L and P function as the RNA polymerase complex, responsible for replicating and transcribing the viral genome. To catalyze the RNA synthesis in both replication and transcription, L sequentially consists of five domains: the RNA-dependent RNA polymerase domain (RdRp), polyribonucleotidyl transferase domain (PRNTase), connector domain (CD), methyltransferase domain (MTase), and C-terminal domain (CTD). P harbors an oligomerization domain (POD) for self-oligomerization, and the oligomeric P attaches to RdRp of L, tethering the polymerase to NC to extract the RNA strand for both replication and transcription. Here, we resolved two L–P complex conformations from the mumps virus (MuV), a typical member of nsNSVs, via cryogenic-electron microscopy.

RdRp-PRNTase is quite conserved in structure amongst nsNSVs, while CD-MTase-CTD resembles an appendage of RdRp-PRNTase with great structural diversity. In MuV Lintegral–P, the appendage is also less resolved compared with the body. Different from the conserved RdRp-PRNTase, CD-MTase-CTD of MuV Lintegral–P adopts a spatial organization distinct from those of PIV-5, though their individual structures are pretty similar. The detailed alignment showed that MTase and CTD in MuV Lintegral–P appears as an integral on the PRNTase side instead of the RdRp side compared with PIV-5 L. The overall spatial organization of CD-MTase-CTD in MuV Lintegral–P is surprisingly similar to VSIV L. VSIV CD-MTase-CTD is highly flexible unless unphosphorylated P locks their configuration, while in MuV, no P fragment is resolved around the appendage. In MuV Lintegral–P, an α-helix hinge termed Hinge-1 (L1416–1431) connecting PRNTase and CD has been visualized. It is supposed to provide flexibility to CD positioning via loops flanking it. Compared with PIV-5, the spatial organization of MuV CD-MTase-CTD renders the helices α53 (L1439–1458) and α57 (L1535–1544) of CD rotating upward and leaves more space for RNA to access MTase. Actually, MuV Lintegral–P forms a continuous positively-charged tunnel from the GDN to the K-D-K-E motifs, ideal for the RNA synthesis followed by 5’ capping and methylation, which is favorable as the transcription state.

> MAGLNEILLPEVHLNSPIVRYKLFYYILHGQLPNDLEPDDLGPLANQNWKAIRAEESQVHARLKQIRVELIARIPSLRWTRSQREIAILIWPRILPILQAYDLRQSMQLPTVWEKLTQSTVNLISDGLERVVLHISNQLTGKPNLFTRSRAGQDTKDYSIPSTRELSQIWFNNEWSGSVKTWLMIKYRMRQLITNQKTGELTDLVTIVDTRSTLCIITPELVALYSSEHKALTYLTFEMVLMVTDMLEGRLNVSSLCTASHYLSPLKKRIEVLLTLVDDLALLMGDKVYGIVSSLESFVYAQLQYGDPVIDIKGTFYGFICNEILDLLTEDNIFTEEEANKVLLDLTSQFDNLSPDLTAELLCIMRLWGHPTLTASQAASKVRESMCAPKVLDFQTIMKTLAFFHAILINGYRRSHNGIWPPTTLHGNAPKSLIEMRHDNSELKYEYVLKNWKSISMLRIHKCFDASPDEDLSIFMKDKAISCPRQDWMGVFRRSLIKQRYRDANRPLPQPFNRRLLLNFLEDDRFDPIKELEYVTSGEYLRDPEFCASYSLKEKEIKATGRIFAKMTKRMRSCQVIAESLLANHAGKLMRENGVVLDQLKLTKSLLTMNQIGIISEHSRRSTADNMTLAHSGSNKHRINNSQFKKNKDNKHEMPDDGFEIAACFLTTDLTKYCLNWRYQVIIPFARTLNSMYGIPHLFEWIHLRLMRSTLYVGDPFNPPSDPTQLDLDTALNDDIFIVSPRGGIEGLCQKLWTMISISTIILSATEANTRVMSMVQGDNQAIAITTRVVRSLSHSEKKEQAYKASKLFFERLRANNHGIGHHLKEQETILSSDFFIYSKRVFYKGRILTQALKNVSKMCLTADILGDCSQASCSNLATTVMRLTENGVEKDLCYFLNAFMTIRQLCYDLVFPQTKSLSQDITNAYLNHPILISRLCLLPSQLGGLNFLSCSRLFNRNIGDPLVSAIADVKRLIKAGCLDIWVLYNILGRRPGKGKWSTLAADPYTLNIDYLVPSTTFLKKHAQYTLMERSVNPMLRGVFSENAAEEEEELAQYLLDREVVMPRVAHVILAQSSCGRRKQIQGYLDSTRTIIRYSLEVRPLSAKKLNTVIEYNLLYLSYNLEIIEKPNIVQPFLNAINVDTCSIDIARSLRKLSWATLLNGRPIEGLETPDPIELVHGCLIIGSDECEHCSSGDDKFTWFFLPKGIRLDDDPASNPPIRVPYIGSKTDERRVASMAYIKGASVSLKSALRLAGVYIWAFGDTEESWQDAYELASTRVNLTLEQLQSLTPLPTSANLVHRLDDGTTQLKFTPASSYAFSSFVHISNDCQILEIDDQVTDSNLIYQQVMITGLALIETWNNPPINFSVYETTLHLHTGSSCCIRPVESCVVNPPLLPVPLINVPQMNKFVYDPEPLSLLEMEKIEDIAYQTRIGGLDQIPLLEKIPLLAHLTAKQMVNSITGLDEATSIMNDAVVQADYTSNWISECCYTYIDSVFVYSGWALLLELSYQMYYLRIQGIQGILDYVYMTLRRIPGMAITGISSTISHPRILRRCINLDVIAPINSPHIASLDYTKLSIDAVMWGTKQVLTNISQGIDYEIVVPSESQLTLSDRVLNLVARKLSLLAIIWANYNYPPKVKGMSPEDKCQALTTHLLQTVEYVEYIQIEKTNIRRMIIEPKLTAYPSNLFYLSRKLLNAIRDSEEGQFLIASYYNSFGYLEPILMESKIFNLSSSESASLTEFDFILNLELSDASLEKYSLPSLLMTAENMDNPFPQPPLHHVLRPLGLSSTSWYKTISVLNYISHMKISDGAHLYLAEGSGASMSLIETFLPGETIWYNSLFNSGENPPQRNFAPLPTQFIESVPYRLIQAGIAAGNGIVQSFYPLWNGNSDITDLSTKTSVEYIIHKVGADTCALVHVDLEGVPGSMNSMLERAQVHALLITVTVLKPGGLLILKASWEPFNRFSFLLTVLWQFFSTIRILRSSYSDPNNHEVYIIATLAVDPTTSSFTTALNRARTLNEQGFSLIPPELVSEYWRKRVEQGQIIQDCIDKVISECVRDQYLADNNIILQAGGTPSTRKWLDLPDYSSFNELQSEMARLITIHLKEVIEILKGQASDHDTLLFTSYNVGPLGKINTILRLIVERILMYTVRNWCILPTQTRLTLRQSIELGEFRLRDVITPMEILKLSPNRKYLKSALNQSTFNHLMGETSDILLNRAYQKRIWKAIGCVIYCFGLLTPDVEGSERIDVDNDIPDYDIHGDII> GAQ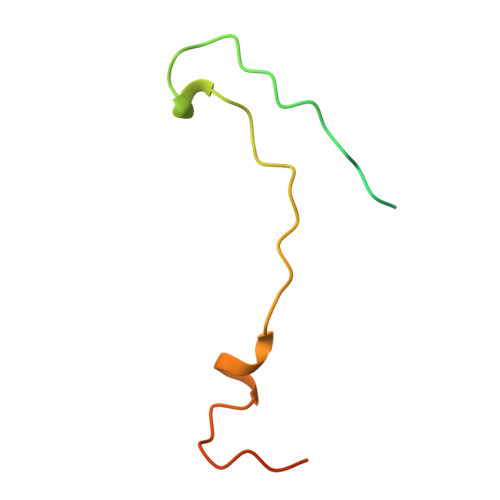LSRNTAGSHTTQTYATGGSTINYNNINYYSHAASAAQNKQDFTQDPSKFTQPIADVIKETAVPLK2-[4-[4-pentyl-3-[(1~{S},2~{R})-2-pyridin-2-ylcyclopropyl]phenyl]phenyl]sulfonylethanol | C27 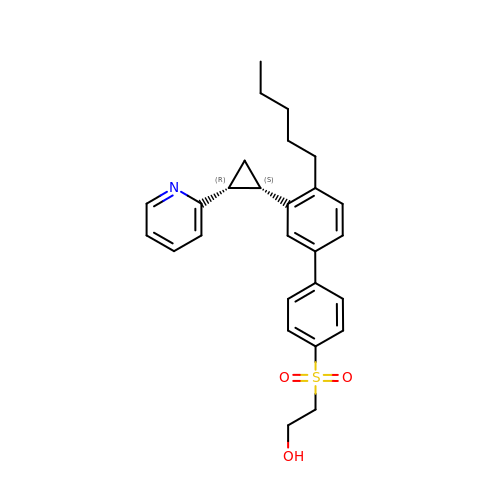H31 N O3 S | RINDEJMEOMKHPC-CLJLJLNGSA-N The exo-β-1,3-galactanase is a glycoside hydrolase from the basidiomycete Phanerochaete chrysosporium (Pc1,3Gal43A), which specifically cleaves AGPs. In this context, exo-β-1,3-galactanase (EC 3.2.1.145) specifically cleaves the nonreducing end β-1,3–linked galactosyl linkage of β-1,3-galactans to release d-galactose (Gal). In this study, we solved the apo and liganded structures of Pc1,3Gal43A, which reveal a glycoside hydrolase family 43 subfamily 24 (GH43_sub24) catalytic domain together with a carbohydrate-binding module family 35 (CBM35) binding domain. The N-terminal catalytic domain consists of a five-bladed β-propeller (Gln21–Gly325), as in other GH clan-F enzymes, and the C-terminal domain (PcCBM35) takes a β-jellyroll fold (Thr326–Tyr448) structure, as in previously reported CBM35s.

In the structure of WT_Gal, one Gal was found at subsite −1, taking a 4C1 chair conformation with α-anomeric conformation of the C-1 hydroxyl group (data not shown). The binding mode of Gal−1 is almost the same as that in E208Q_Gal3, but the C-1 hydroxyl group in the axial position forms hydrogen bonds with Gly228 and Gln263. Comparison of the Gal-bond structure (i.e. WT_Gal) with the Gal3-bond structure (i.e. E208Q_Gal3) showed that the fluctuations of Glu(Gln)208, Asn179, and Thr226 of E208Q_Gal3 were smaller than these in WT_Gal. Therefore, it can be inferred that these residues recognize the ligands at the plus subsites. The catalytic acid, Glu208, has two major conformations in WT and WT_Gal. Thus, the movement of this residue appears to be important for catalysis. Asp158 of WT and E208A_Gal3 show greater vibration than WT_Gal and E208Q_Gal3. The role of Asp158 is thought to be a pKa modulator; therefore, its function and conformational stability might be related.

> NQIVSGAAWTDTAGNTIQAHGAGILQVGSTFYWFGEDKSHNSALFKAVSCYTSSDLVNWSRQNDALSPIAGTMISTSNVVERPKVIFNQKNSEYVMWFHSDSSNYGAAMVGVATAKTPCGPYTYKGSFKPLGADSRDESIFQDDDSAQTAYLLYASDNNQNFKISRLDANYYNVTAQVSVMNGATLEAPGIVKHNGEYFLIASHTSGWAPNPNKWFSASSLAGPWSAQQDIAPSATRTWYSQNAFDLPLGSNAIYMGDRWRPSLLGSSRYIWYPLDFSSGAPQIVHADVWSVNVQAGTYSVASGTSYEAENGQRGGSSTILSGSGFSGGKAVGYLGHGGTVTINNVQSNGGSHWVALYFANGDSTYRNVTVSVNGGPSVLVDQPDSGGGNVVISVPVKLNLNSGENSITFGSGQSNYAADLDKIIVY>[4x]ATRSPGVVISDDEPGYDLDLFAIPNHYAEDLERVFIPHGLIMDRTERLARDVMKEMGGHHIVALCVLKGGYKFFADLLDYIKALNRNSDRSI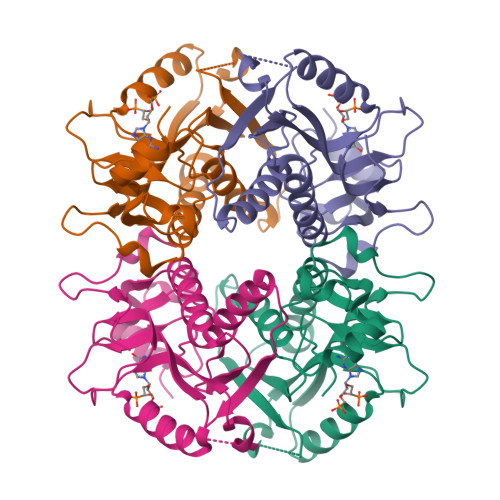PMTVDFIRLKSYANDQSTGDIKVIGGDDLSTLTGKNVLIVEDIIDTGKTMQTLLSLVRQYNPKMVKVASLLVKRTPRSVGYKPDFVGFEIPDKFVVGYALDYNEYFRDLNHVAVISETGKAKYKA> MGKIFEDNSLTIGHTPLVRLNRIGNGRILAKVESRNPSFSVKCRIGANMIWDAEKRGVLKPGVELVEPTSGNTGIALAYVAAARGYKLTLTMPETMSIERRKL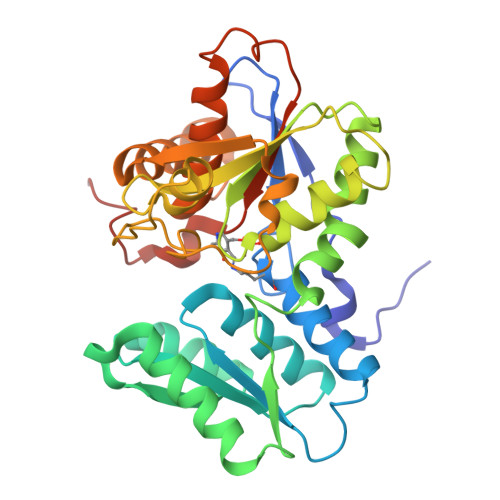LKALGANLVLTEGAKGMKGAIQKAEEIVASNPEKYLLLQQFSNPANPEIHEKTTGPEIWEDTDGQVDVFIAGVGTGGTLTGVSRYIKGTKGKTDLISVAVEPTDSPVIAQALAGEEIKPGPHKIQGIGAGFIPANLDLKLVDKVIGITNEEAISTARRLMEEEGILAGISSGAAVAAALKLQEDESFTNKNIVVILPSSGERYLSTALFADLFTEKELQQ> MPERDALLTDLVGDRAAEWDTSGELPRDLLVRLGADGLLCAEVAAEHGGLGL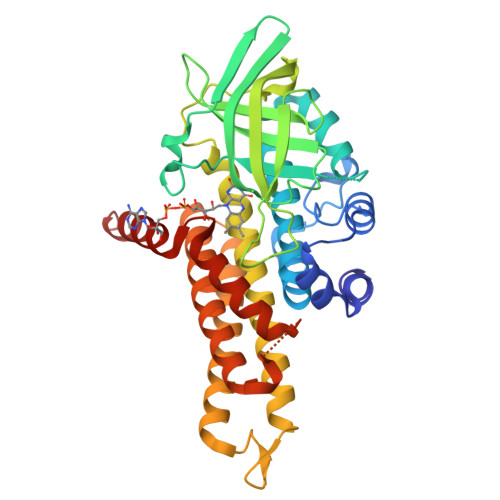GSRENGEFTAHVGSLCSSLRSVMTSQGMAAWTVQRLGDAGQRATFLKELTSGKLAAVGFSERQAGSDLSAMRTRVRLDGDTAVVDGHKVWTTAAAYADHLVVFGLQEDGSGAVVVVPADTPGVRVERVPKPSGCRAAGHADLHLDQVRVPAGAVLAGSGASLPMLVAASLAYGRKSVAWGCVGILRACRTAAVAHARTREQFGRPLGDHQLVAGHIADLWTAEQIAARVCEYASDHWDEGSPEMVPATILAKHVAAERAAAGAATAAQVLASAGAREGHVVERAYRDAKLMEIIEGSSEMCRVMLAQHALALPA> GPHMSTSS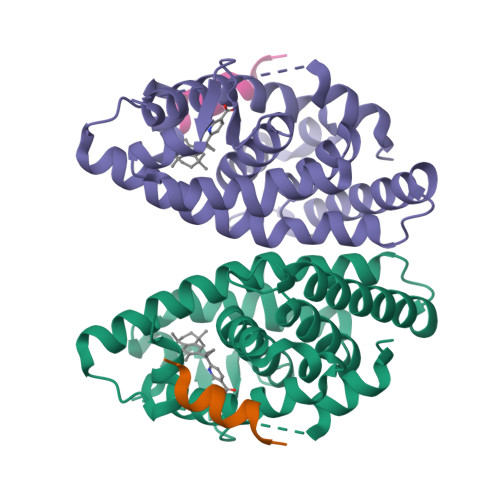ANEDMPVEKILEAELAVEPKTETYVEANMGLNPSSPNDPVTNICQAADKQLFTLVEWAKRIPHFSELPLDDQVILLRAGWNELLIASFSHESIAVKDGILLATGLHVHRNSAHSAGVGAIFDRVLTELVSKMRDMQMDKTELGCLRAIVLFNPDSKGLSNPAEVEALREKVYASLEAYCKHKYPEQPGRFAKLLLRLPALRSIGLKQLEHLFFFKLIGDTPIDTFLMEMLEAPHQAT;> KHKILHRLLQDSS> PFVNKQFNYKDPVNGVDIAYIKIPNAGQMQPVKAFKIHNKIWVIPERDTFTNPEEGDLNPPPEAKQVPVSYYDSTYLSTDNEKDNYLKGVTKLFERIYSTDLGRMLLTSIVRGIPFWGGSTIDTELKVIDTNCINVIQPDGSYRSEELNLVIIGPSADIIQFECKSFGHEVLNLTRNGYGSTQYIRFSPDFTFGFEESLEVDTNPLLGAGKFATDPAVTLAHQLIHAGHRLYGIAINPNRVFKVNTNAYYEMSGLEVSFEELRTFGGHDAKFIDSLQENEFRLYYYNKFKDIASTLNKAKSIVGTTASLQYMKNVFKEKYLLSEDTSGKFSVDKLK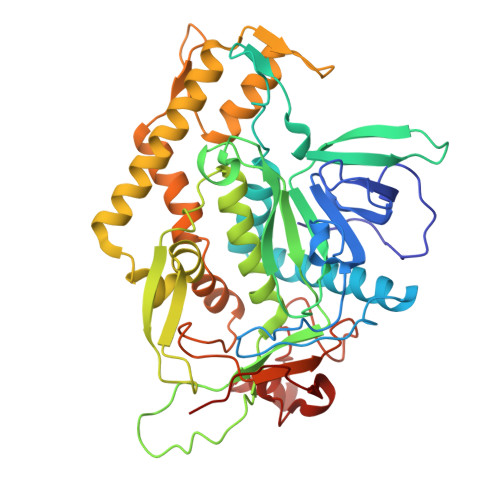FDKLYKMLTEIYTEDNFVKFFKVLNRKTFLNFDKAVFKINIVPKVNYTIYDGFNLRNTNLAANFNGQNTEINNMNFTKLKNFTPLVPR>MLEINKIHQMNCFDFLDQVENKSVQLAVIDPPYNLSK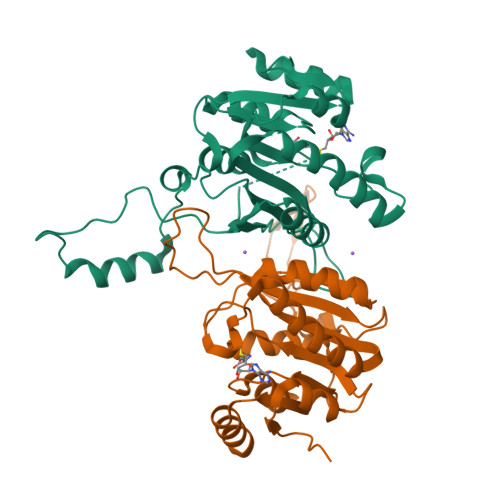ADWDSFDSHNEFLAFTYRWIDKVLDKLDKDGSLYIFNTPFNCAFICQYLVSKGMIFQNWITWDKRDGMGSAKRRFSTGQETILFFSKSKNHTFNYDEVRVPYESTDRIKHASEKGILKNGKRWFPNPNGRLCGEVWHFSSQRHKEKVNGKTVKLTHITPKPRDLIERIIRASSNPNDLVLDCFMGSGTTAIVAKKLGRNFIGCDMNAEYVNQANFVLNQLEIN[2x]> TSFTRNIVGRDGLCVDVRNGYDTDGTPLQLWPCGTQR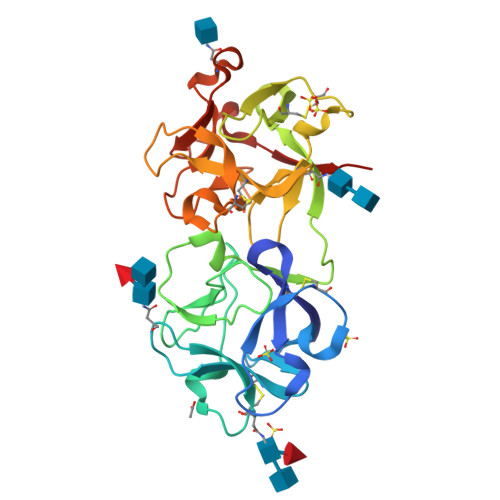NQRWTFDSDDTIRSMGKCMTANGLNNGSNIVIFNCSTAAENAIKWEVPIDGSIINPSSGLVMTAPRAASRTILLLEDNIYAASQGWTVTNNVKPIVASIVGYKEMCLQSNGENNGVWMEDCEATSLQQQWALYGDRTIRVNSTRGLCVTTNGYNSKDLIIILKCQGLPSQRWFFNSDGAIVNPKSRLVMDVRASNVSLREIIIFPATGNPNQQWVTQVLPS> GHFKDPKRLYCKNGGFFLRIHPDGRVDGVREKSDPHIKL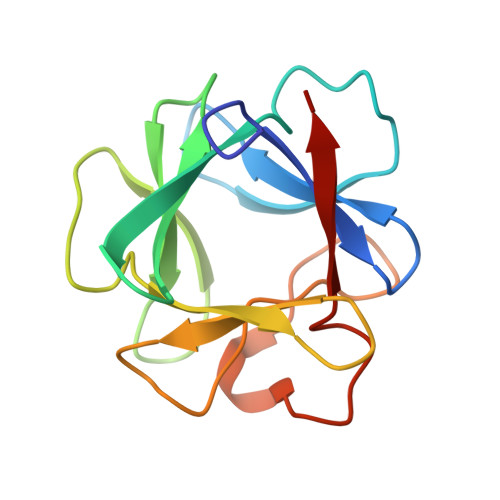QLQAEERGVVSIKGVSANRYLAMKEDGRLLASKSVTDECFFFERLESNNYNTYRSRKYTSWYVALKRTGQYKLGSKTGPGQKAILFLPMSAKS> MSDSEGGLASEVEHEKRSRSTSNRPNYAIDTEDLDIDENDENEDDDYREEEANEGVNEEEISDEEEQINKSGRNKRRHVDEEED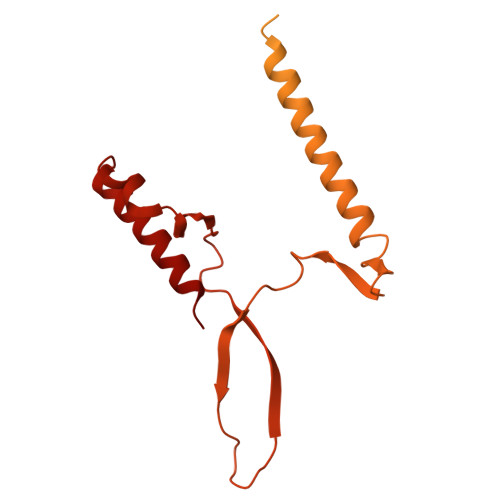LSEDKGVTRSRNRSKFKKPVFPGIDDAEENLNPLKVVNEEYVLPDDPEGETKITADGDLLGGREFLVRTFTLTEKGNRKFMLATEPARIVGFRDSYLFFQTHPNLYKFILNQTQKNDLIDRGVLPYSYRNRQIALVTARGVFKEFGAKIIRGGKHITDDYYASELRTKGNVIEGKLAGDPIDKSARALETMMYPASENGINPAKNQVEFFEHRPHGHMSNSNIIASGSKLSSTNWLYQHSAACSRFNSDLFYDRVKVLLVDQQGLRDAYTNILHIPESTQSTTVLGWRRSKNDSPSDTSIVYETVIHDNDLNKPKTGLSEIPKEIYEDVVDEDVLRAITEQQNFEKCNEYI>MERYESLFAQLKERKEGAFVPFVTLGDPGIEQSLKIIDTLIEAGADALELGIPFSDPLADGPTIQNATLRAFAAGVTPAQCFEMLALIREKHPTIPIGLLMYANLVFNKGIDEFYARCEKVG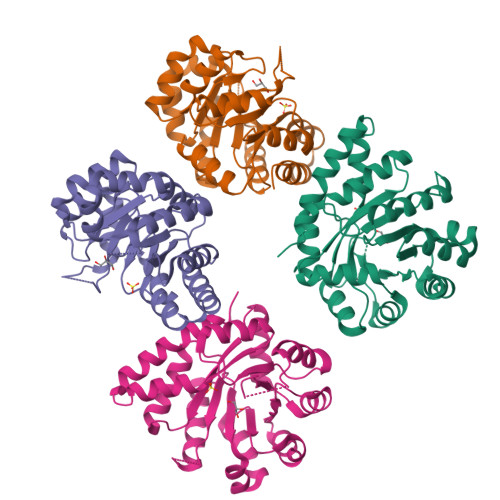VDSVLVADVPVEESAPFRQAALRHNVAPIFICPPNADDDLLRQIASYGRGYTYLLSRAGVTGAENRAALPLNHLVAKLKEYNAAPPLQGFGISAPDQVKAAIDAGAAGAISGSAIVKIIEQHINEPEKMLAALKVFVQPMKAATRS[2x]>SMAKNRRDRNSWGGFSEKTYEWSSEEEEPVKKAGPVQVLIVKDDHSFELDETALNRILLSEAVRDKEVVAVSVAGAFAKGKSFLMDFMLRYMYNQESVDWVGDYNEPLTGFSWRGGSERETTGIQIWSEIFLINKPDGKKVAVLLMDTQGTFDSQSTLRDSATVFALSTMISSIQVYNLSQNVQEDDLQHLQLFTEYGRLAMEETFLKPFQSLIFLVRDWSFPYEFSYGADGGAKFLEKRLKVSGNQHEELQNVRKHIHSCFTNISCFLL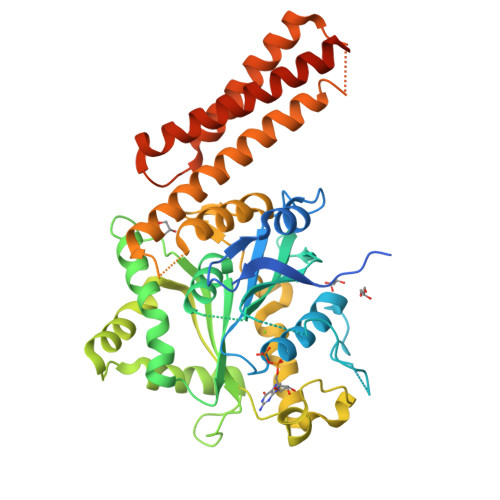PHPGLKVATNPNFDGKLKEIDDEFIKNLKILIPWLLSPESLDIKEINGNKITCRGLVEYFKAYIKIYQGEELPHPKSMLQATAEANNLAAVATAKDTYNKKMEEICGGDKPFLAPNDLQTKHLQLKEESVKLFRGVKKMGGEEFSRRYLQQLESEIDELYIQYIKHNDSKNIFHAARAAALEHHHHHH[2x]>KPRKARTAFSDHQLNQLERSFERQKYLSVQDRMDLAAALNLTDTQVKTWYQNRRTKWKRQTA[4x]

Transcription factors (TFs) recognize specific bases within their DNA-binding motifs, with each base contributing nearly independently to total binding energy. However, the energetic contributions of particular dinucleotides can deviate strongly from the additive approximation, indicating that some TFs can specifically recognize DNA dinucleotides. Here we solved high-resolution (<1 Å) structures of MYF5 and BARHL2 bound to DNAs containing sets of dinucleotides that have different affinities to the proteins. The dinucleotides were recognized either enthalpically, by an extensive water network that connects the adjacent bases to the TF, or entropically, by a hydrophobic patch that maintained interfacial water mobility.

The molecular interactions observed in the structure of BARHL2 bound to DNATT, which showed the next highest affinity in the SELEX experiments, were strikingly different from those of BARHL2–DNAAC. The extensive water network is lost because of a hydrophobic patch in the major groove, formed by the methyl groups of the two Ts. The hydrophobic contact with Thr285 is replaced by hydrophobic contact between the methyl group (CG2) of Thr278 and C7 of the first T (T7) of TT. Only one water connecting the side-chain oxygen of Thr285 with the side-chain oxygen of Asn282 was observed in the region around Thr285. On the other side, Asn282 is connected to O4 of T7 through one water and to O4 of the second T (T8) of TT through a water chain containing three molecules. Thus, most of the contacts in the complex BARHL2–DNATT are shifted from the Thr285 region to the Thr278. An additional observation is that the side chain of Arg289 forms a hydrophobic contact with the methyl group of Thr285, in contrast to BARHL2–DNAAC, in which Arg289 shows two conformations, both of which are turned away from Thr285. The number of low-mobility water molecules observed at the protein–DNA interface was significantly greater for BARHL2–DNAAC than BARHL2–DNATT. Consistent with the relatively high predicted mobility of these waters, the level of electron density seen in crystal structure of the BARHL2–DNATT complex in this region (<1σ) appears similar to that of free solvent at the limit of resolution (1.85 Å), thus explaining why only few water molecules are seen in BARHL2–DNATT crystal structure at the dinucleotide recognition site. By contrast, the TT dinucleotide exposes a more hydrophobic surface to solvent molecules in the major groove, which leads to a more mobile water network at the complex interface that is entropically more favorable than that of the AC dinucleotide.>[4x]MEAGITGTWYNQLGSTFIVTAGADGALTGTYVTA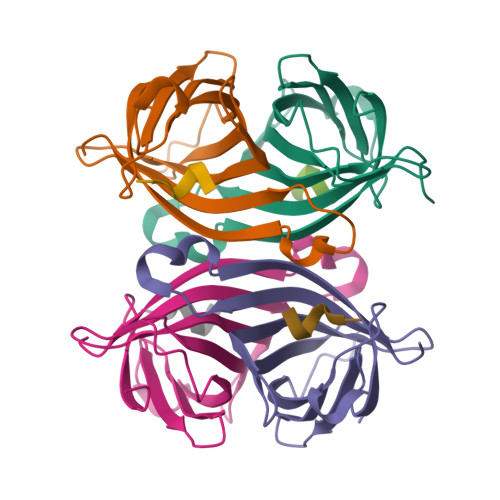RGNAESRYVLTGRYDSAPATDGSGTALGWTVAWKNNYRNAHSATTWSGQYVGGAEARINTQWLLTSGTTEANAWKSTLVGHDTFTKVKPSAAS;>[4x]NWSHPQFEK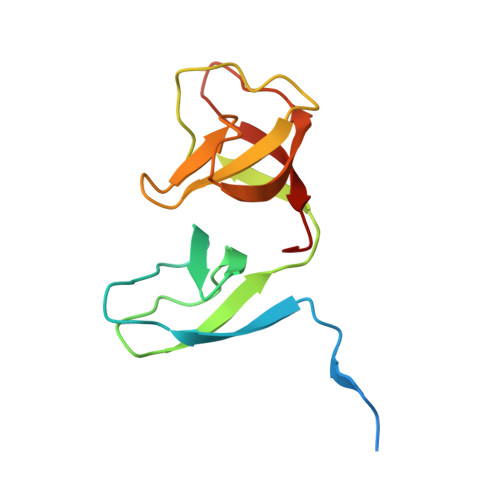> MAFKGQPTPSTITQITRAKISDGKSVRVILSEGESTKTQQFYLINGFFGVAMQDGEKGDEVTLQIEQAEYETDNIVTSEAFEAGKLIYWDNTAKKFTTTSASNRLVGRVTDGKDSNNVIWFILLPQQ>QLTPRRPYLLRAFYEWLLDNQLTPHLVVDVTLPGVQVPMEYARDGQIVLNIAPRAVGNLELANDEVRFNARFGGIPRQVSVPLAAVLAIYARENGAGTMFEP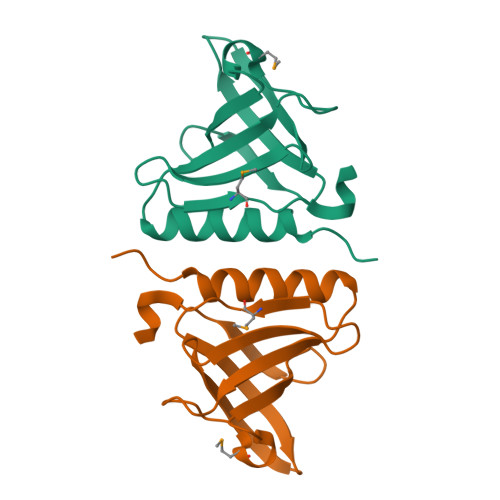EAAYD[2x]> VEEILEKALELVIPDEEEVRKGREAEEELRRRL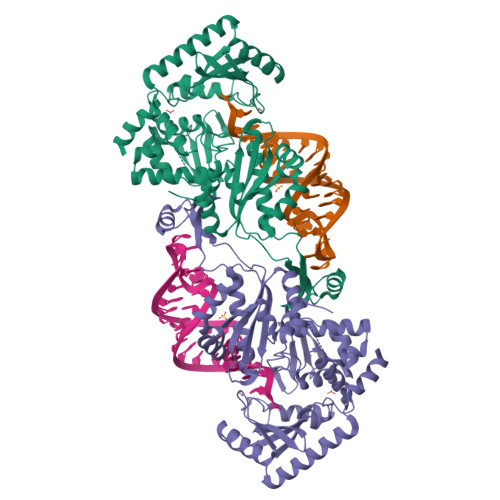DELGVEYVFVGSYARNTWLKGSLEIDVFLLFPEEFSKEELRERGLEIGKAVLDSYEIRYAEHPYVHGVVKGVEVDVVPCYKLKEPKNIKSAVDRTPFHHKWLEGRIKGKENEVRLLKGFLKANGIYGAEYKVRGFSGYLCELLIVFYGSFLETVKNARRWTRRTVIDVAKGEVRKGEEFFVVDPVDEKRNVAANLSLDNLARFVHLCREFMEAPSLGFFKPKHPLEIEPERLRKIVEERGTAVFAVKFRKPDIVDDNLYPQLERASRKIFEFLERENFMPLRSAFKASEEFCYLLFECQIKEISRVFRRMGPQFEDERNVKKFLSRNRAFRPFIENGRWWAFEMRKFTTPEEGVRSYASTHWHTLGKNVGESIREYFEIISGEKLFKEPVTAELCEMMGVKD> MAKVLCVLYDDPVDGYPKTYARDDLPKIDHYPGGQTLPTPKAIDFT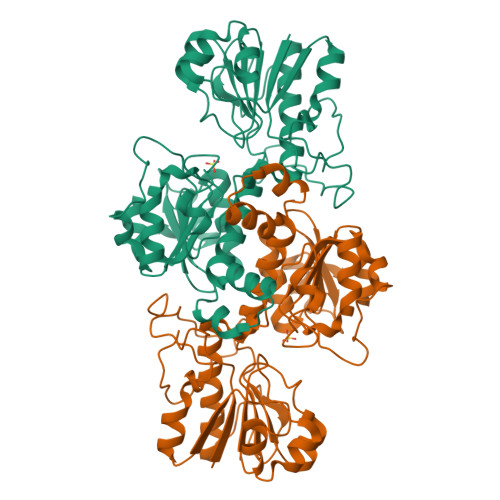PGQLLGSVSGELGLRKYLESNGHTLVVTSDKDGPDSVFERELVDADVVISQPFWPAYLTPERIAKAKNLKLALTAGIGSDHVDLQSAIDRNVTVAEVTYCNSISVAEHVVMMILSLVRNYLPSHEWARKGGWNIADCVSHAYDLEAMHVGTVAAGRIGLAVLRRLAPFDVHLHYTDRHRLPESVEKELNLTWHATREDMYPVCDVVTLNCPLHPETEHMINDETLKLFKRGAYIVNTARGKLCDRDAVARALESGRLAGYAGDVWFPQPAPKDHPWRTMPYNGMTPHISGTTLTAQARYAAGTREILECFFEGRPIRDEYLIVQGGALAGTGAHSYSKGNATGGSEEAAKFKKAV>[4x]MMMKFINIGYGNMVSAARIITIVSPDSAPIKRIIQDAREKGKLVDATHGRRTRAVI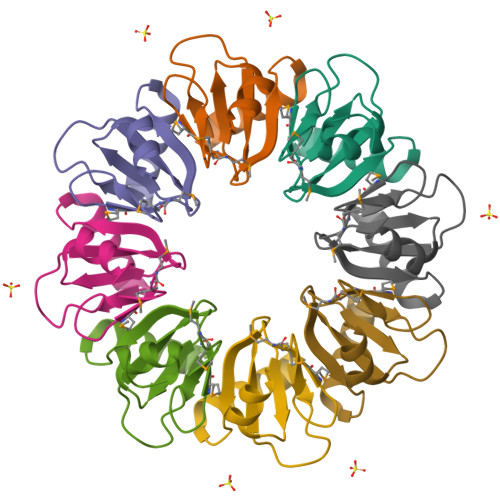ITDSDHVILSSVQPETVANRLYGSDDFSEEG> MGSRSSHAAVIPDGDSIRRETGFSQASLLRLHHRFRALDRNKKGYLSRMDLQQIGALAVNPLGDRIIESFFPDGSQRVDFPGFVRVLAHFRPVEDEDTETQDPKKPEPLNSRRNKLHYAFQLYDLDRDGKISRHEMLQVLRLMVGVQVTEEQLENIADRTVQEADEDGDGAVSFVEFTKS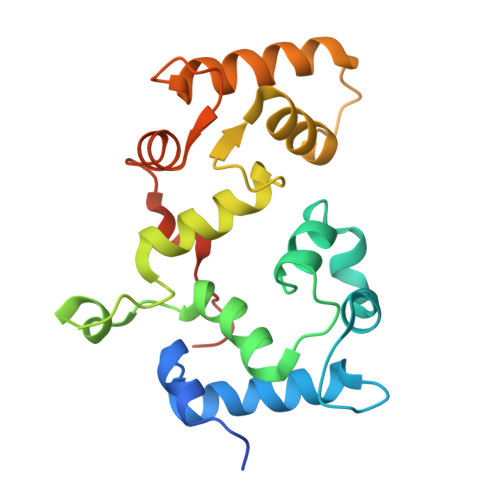LEKMDVEQKMSIRILKHHHHHH>[4x]GAGEARLEEAVNRWVLKFYFHEALRAFRGSRYGDFRQIRDIMQALLVRPLGKEHTVSR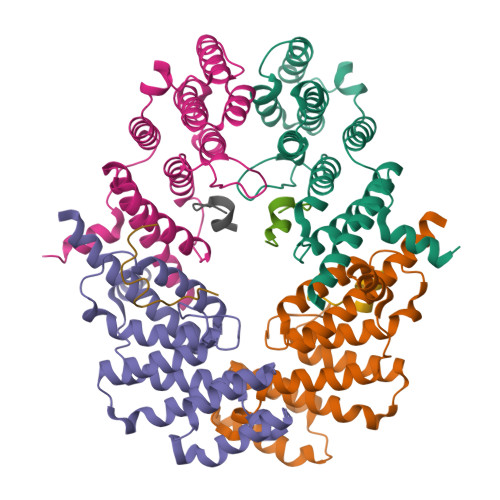LLRVMQCLSRIEEGENLDCSFDMEAELTPLESAINVLEMIKTEFTLTEAVVESSRKLVKEAAVIICIKNKEFEKASKILKKHMSKDPTTQKLRNDLLNIIREKNLAHPVIQNFSYETFQQKMLRFLESHLDDAEPYLLTMAKKALK;>SEFRGLALKYLLTPVNFFQAGYSSRRFDQQVEKYHK[4x]>[2x]GSAPYASLTEIEHLVQSVCKSYRETCQLRLEDLLRQRSNIFSREEVTGYQRKSMWEMWERCAHHLTEAI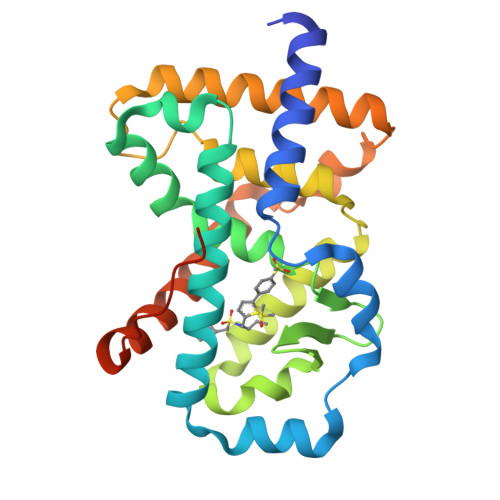QYVVEFAKRLSGFMELCQNDQIVLLKAGAMEVVLVRMCRAYNADNRTVFFEGKYGGMELFRALGCSELISSIFDFSHSLSALHFSEDEIALYTALVLINAHRPGLQEKRKVEQLQYNLELAFHHHLCKTHRQSILAKLPPKGKLRSLCSQHVERLQIFQHLHPIVVQAAFPPLYKELFSGNS> 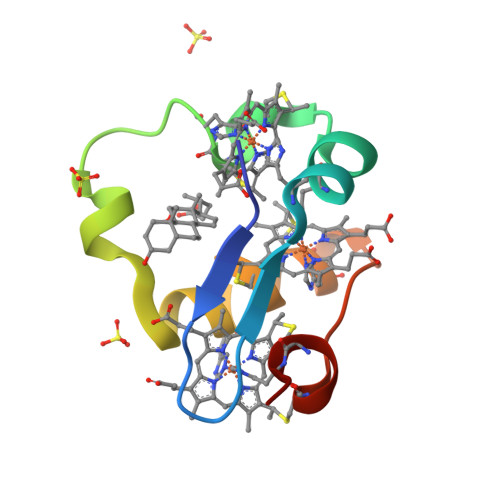ADDIVLKAKNGDAKFPHKAHQKAVPDCKKCHEKGPGKIEGFGKEMAHGKGCKGCHEEMKKGPTKCGECHKK> MNVQDRRRLLGPAAAKPMAFSNTTTHVPEKKSTDLTPKGNESEQELSLHTGFIENCNGSALVEARSLGHQTSLITAVYGPRSIRGSFTSQGTISIQLKNGLLEKYNTNELKEVSSFLMGIFNSVVNLSRYPKSGIDI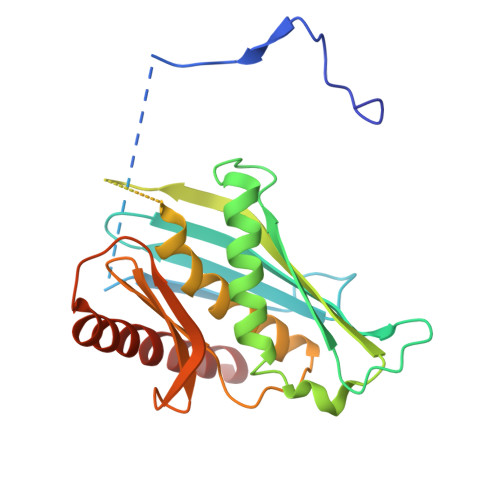FVYLTYDKDLTNNPQDDDSQSKMTSSQISSLIPHCITSITLALADAGIELVDMAGAGEANGTVVSFIKNGEEIVGFWKDDGDDEDLLECLDRCKEQYNRYRDLMISCLMNQET> MRGSHHHHHHGSVIFDKRIKDEEDVEKELGLPVLGSIQKFNMSKKENTTTTLFVYEKPKSTISEKFRGIRSNIMFSKANGEVKRLLVTSEKPGAGKSTVVSNVAITYAQAGYKTLVIDGDMRKPTQNYIFNEQNNNGLSSLIIGRTTMSEAITSTEIENLDLLTAGPVPPNPSELIGSERFKELVDLFNKRYDIIIVDTPPVNTVTDAQLYARAIKDSLLVIDNEKNDKNEVKKAKALMEKAGSNILGVILNKTKVDKSSSYYHYYGDE

A new family of protein tyrosine-kinases harboring a P-loop type nucleotide binding-domain with a Walker A motif has been described. They have been called BY-kinases (Bacterial-tyrosine-kinases) as they are only found in bacterial genomes. BY-kinase autophosphorylation on a C-terminal tyrosine cluster, called Y-cluster is crucial in regulating polysaccharide export. In firmicutes, the situation is quite similar except that BY-kinases are split into two proteins: one corresponds to the cytoplasmic catalytic domain of proteobacterial BY-kinases (about 230 residues) and the other is a transmembrane domain homologous to the Wzz-like domain (about 230 residues) of proteobacterial BY-kinases.

To test this and further understand why CapB1 is less active than CapB2, we solved the crystal structure of the CapA1B1 chimera. Clear electron density corresponding to a bound ADP molecule and associated Mg2+ ion was observed in the active site of CapA1B1. Despite the presence of the bound nucleotide, CapB1 residues 1 to 8 as well as the CapA1 last residue Asn222 are disordered. The stacking interaction between the CapA1 Phe221 and the base part of the bound ADP is conserved. Phe221 is stabilized in this position by a T-shaped hydrophobic interaction with CapB1 residue Phe12 replacing the stacking interaction with CapB2 residue Ile12 observed in the CapA1B2 structure. Surprisingly, despite the inactivity of the protein, the CapA1B1 structure does not display the expected octameric conformation and the Y-cluster is disordered. This suggests that CapB1 is intrinsically in the monomeric active conformation compatible with the binding of specific protein substrate. The basic isoelectric point of CapB1, with a calculated value of 8.8 (compared with 5.45 for CapB2), suggests that the formation of a CapB1 oligomer compatible with trans-autophosphorylation could be impaired by unfavorable electrostatic surface charges. Altogether, this data prove that CapB1 does not possess a tyrosine-kinase activity despite its BY-kinase signature and a 3D structure very similar to that of the active BY-kinase CapB2.>KQFSAMNKFKKMALRVIAESLSEEEIAGLKEMFNMIDADKSGQITFEELKAGLKRVGANLKESEILDLMQAADVDNSGTIDYKEFIAATLHLNKIEREDHLFAAFTY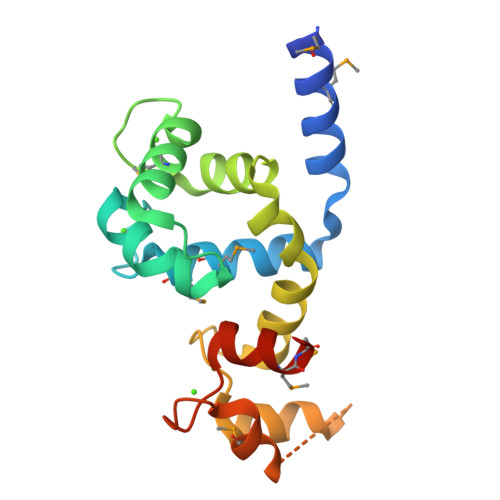FDKDGSGYITPDELQQACEEFGVEDVRIEELMRDVDQDNDGRIDYNEFVAMMQKGSITG[2x]> FENHLISEICPKTRNPSLCLQALESDPRSASKDLKGLGQFSIDIAQASAKQTSKIIASLTNQATDPKLKGRYETCSENYADAIDSLGQAKQFLT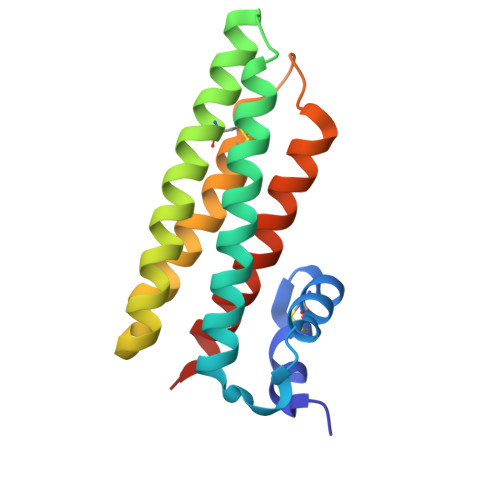SGDYNSLNIYASAAFDGAGTCEDSFEGPPNIPTQLHQADLKLEDLCDIVLVISNLLPGS>AKVKIKPLEDKILVQAGEAETMTPSGLVIPENAKEKPQEGTVVAVGPGRWDEDGAKRIPVDVSEGDIVIYSKYGGTEIKYNGEEYLILSARDVLA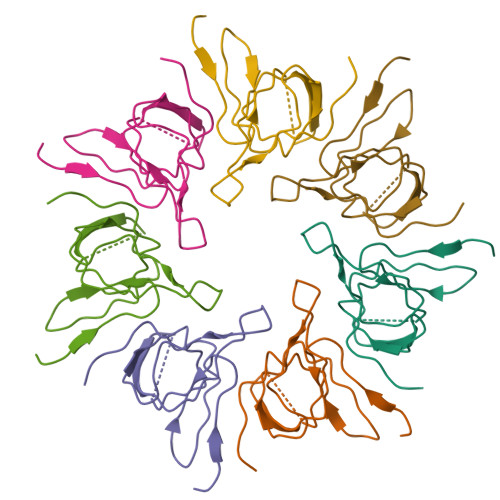VVSK[7x]> MGSSKPLKGFVICCTSIDLKQRTEISTKATKLGAAYRSDFTKDVTHLIAGDFDTPKYKFAAKSRPDIKIMSSEWIPVLYESWVQGEDLDD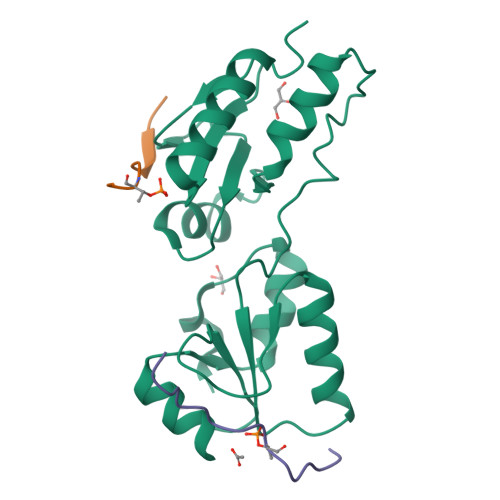GLLVDKHLLPTLFKCRVCLTNIGQPERSRIENYVLKHGGTFCPDLTRDVTHLIAGTSSGRKYEYALKWKINVVCVEWLWQSIQRNAVLEPQYFQLD;>[2x]GYGEVLVPETVAQHRT N-(cyclopent-3-ene-1-carbonyl)-L-histidine | C12 H15 N3 O3 | 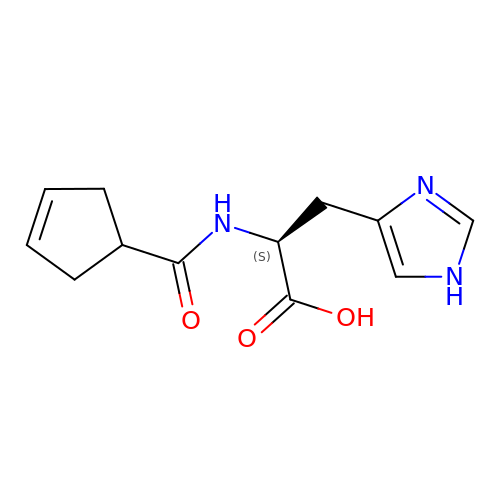SKAVNIUEIPWYLP-JTQLQIEISA-N O2'-METHYLGUANOSINE-5'-MONOPHOSPHATE 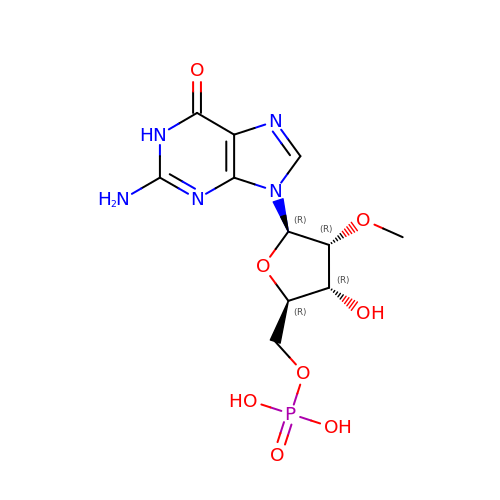| C11 H16 N5 O8 P | YPMKZCOIEXUDSS-KQYNXXCUSA-N>[4x]MIMNLTDKTVLITGGASGIGYAAVQAFLGQQANVVVADIDEAQGEAMVRKENNDRLHFVQTDITDEAACQHAVESAVHTFGGLDVLINNAGIEIVAPIHEMELSDWNKVLQVNLTGMFLMSKHALKHMLAAGKGNIINTCSVGGLVAWPDIPAYNASKGGVLQLTKSMAVDYAKHQIRVNCV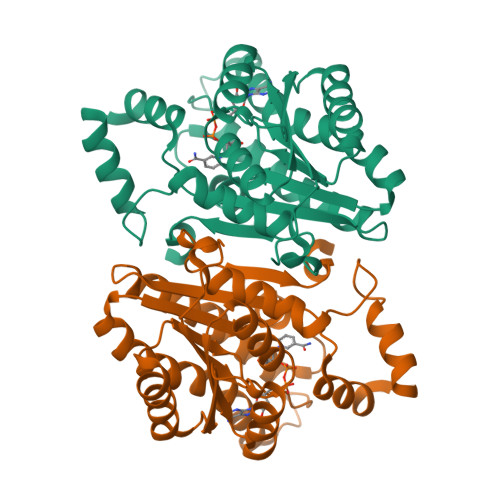CPGIIDTPLNEKSFLENNEGTLEEIKKEKAKVNPLLRLGKPEEIANVMLFLASDLSSYMTGSAITADGGYTAQ>[2x]G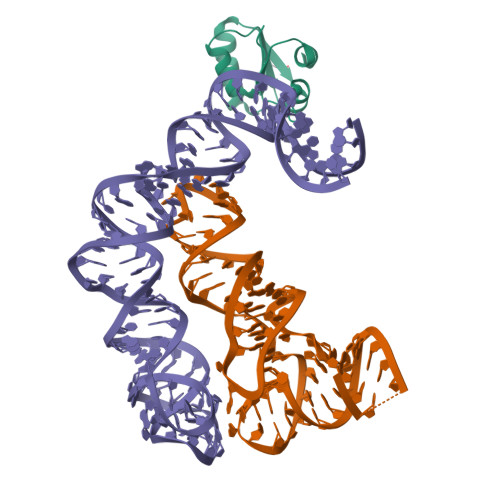SYDKVSQAKSIIIGTKQTVKALKRGSVKEVVVAKDADPILTSSVVSLAEDQGISVSMVESMKKLGKACGIEVGAAAVAIIL> MEKIADSGPVQIFLSRRKLLAFSGASLTVAAIGAPSKGSTQDVVASNRDSISDFMQLSAFATGHKNLDLNIGSALLLAFEAQKHDFSTQIKALREHIT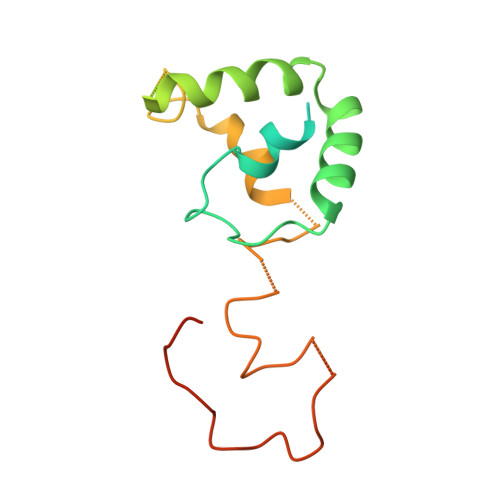KNNYQDVEALDAAMKDDPLHPTLIQIIRAWYSGVIEDETNAKVYAFEKALMYQPSRDVVVIPTYAHNGPNYWVSEPASVDVMPAF>MHHHHHHENLYFQSHQGPEVTLITANAEGIEGGKTTIKSRSVDVGVVESATLADDLTHVEIKARLNSGMEKLLHKDTVFWVVKPQIGREGISGLGTLLSGVYIELQPGAKGSKMDKYDLLDSPPLAPPDAKGIRVILDSKKAGQLSPGDPVLFRGYRVGSVETSTFDTQKRNISYQLFINAPYDRLVTNNVRFWKDSGIAVDLTSAGMRVEMGSLTTLLSGGVSFDVPEGLDLGQPVAPKTAFVLYDDQKSIQDSLYTDHIDYLMFFKDSVRGLQPGAPVEFRGIRLGTVSKVPFFAPNMRQTFNDDYRIPVLIRIEPERLKMQLGENADVVEHLGELLKRGLRGSLKTGNLVTGALYVDLDFYPNTPAITGIREFNGYQIIPTVSGGLAQIQQRLMEALDKINKLXXXXXXXXXXXXXXXXXXXXXXXXXXXXX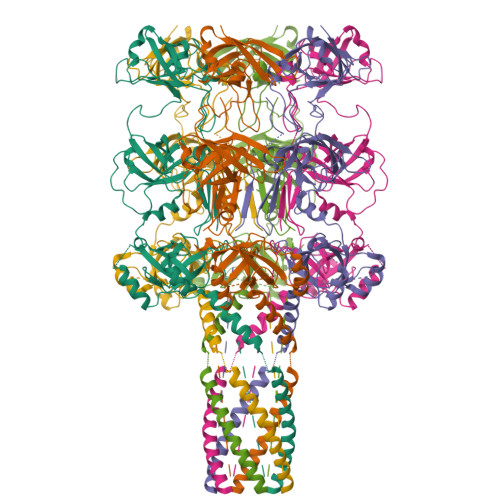XXXXXXXXXXXXXXXXXX[6x]> GSMAWHLGIRSQSRPNDIMAEVCRAIKQLDYEWKVVNPYYLRVRRKNPVTSTFSKMSLQLYQVDSRTYLLDFRSIDDEITEAKSGTATPQRSGSISNYRSCQRSDSDAEAQGKPSEVSLTSSVTSLDSSPVDVAPRPGSHTIEFFEMCANLIKILAQ;> MGPYGQEMYAFRSEERFKSPPILPPHLLQVILNKDTNISCDPALL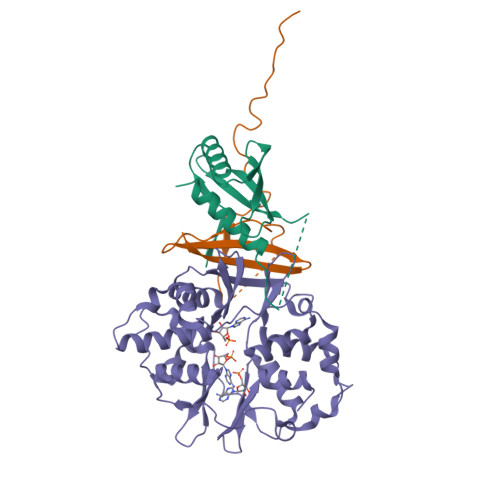PEPNHVMLNHLYALSIKDSVMVLSATHRYKKKYVTTLLYKPI;> MESVAAESAPAPENEHSQETPESNSSVYTTFMKSHRCYDLIPTSSKLVVFDTSLQVKKAFFALVTNGVRAAPLWDSKKQSFVGMLTITDFINILHRYYKSALVQIYELEEHKIETWREVYLQDSFKPLVCISPNASLFDAVSSLIRNKIHRLPVIDPESGNTLYILTHKRILKFLKLFITEFPKPEFMSKSLEELQIGTYANIAMVRTTTPVYVALGIFVQHRVSALPVVDEKGRVVDIYSKFDVINLAAEKTYNNLDVSVTKALQHRSHYFEGVLKCYLHETLEAIINRLVEAEVHRLVVVDEHDVVKGIVSLSDILQALVLTGGEKKP> GPLGSMDPSVKKDEIYYTILNIIQNYFIEYCTGKNRNFHVEDENTYIIVKNMCDIILRDNIVEFRKDIDRCSDIENEIPEIVYDTIHDKITWGRVISIIAFGAYVTKVFKEKGRDNVVDLMPDIITESLLSRCRSWLSDQN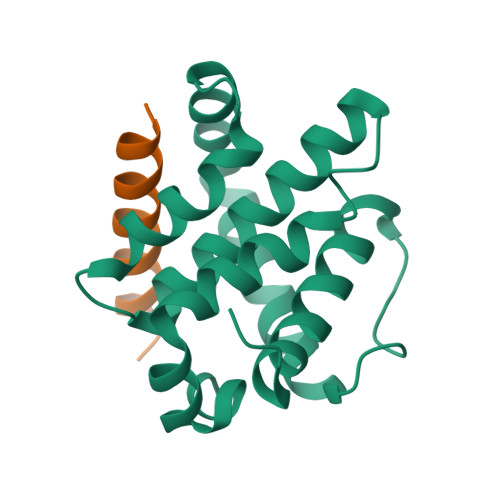CWDGLKA;> DMRPEIWIAQELRRIGDEFNAYYARR>GSHMSAPLPLDELRTFAEVLDRVKAAYVEPVDDKTLLENAIKGMLSNLDPHSAYLGPEDFAELQESTSGEFGGLGIEVGSEDGFIKVVSPIDDTPAARAGIQPGDLIVQIDGKPTKGQSMTEAVDSMRGKAGSPITLTIVRDGGRPFDVELKRAIIKVKSVKSQVLEPGYAYLRITQFQVNTGEEVVKALNQLRKDNKGRLKGLVLDLRNNPGGVLQSAVEVADAFLTKGLIVYTKGRIANSELRFSADPADPSDKVPLVVLINGGSAAAAEIVAGALQDQKRAILMGTDSFGKGSVQTVLPLNNDRALKLTTALYYTPNGRSIQAQGIVPDIEVGRAKVTQERSSFEGFKEADLQGHLANGNGGADRPTGKRAAPSERPQDSDYQLSQALSLLKGLSVTRGN[6x];>MEDTAVETKAKPEKYGSFSEDSLYSLLVAELAGQRNRFDIALSNYVVQAQKTRDPGVSERAFRIAEYLGADQEALDTSLLWARSAPDNLDAQRAAAIQLARAGRYEESMVYMEKVLNGQGDTHFDFLALSAAETDPDTRAGLLQSFDHLLKKYPNNGQLLFGKALLLQQDGRPDEALTLLEDNSASRHEVAPLLLRSRLLQSMKRSDEALPLLKAGIKEHPDDKRVRLAYARLLVEQNRLDDAKAEFAGLVQQFPDDDDLRFSLALVCLEAQAWDEARIYLEELVERDSHVDAAHFNLGRLAEEQKDTARALDEYAQVGPGNDFLPAQLRQTDVLLKAGRVDEAAQRLDKARSEQPDYAIQLYLIEAEALSNNDQQEKAWQAIQEGLKQYPEDLNLLYTRSMLAEKRNDLAQMEKDLRFVIAREPDNAMALNALGYTLADRTTRYGEARELILKAHKLNPDDPAILDSMGWINYRQGKLADAERYLRQALQRYPDHEVAAHLGEVLWAQGRQGDARAIWREYLDKQPDSDVLRRTIKRLTGAETP[3x]

During bacterial cell growth, hydrolases cleave peptide cross-links between strands of the peptidoglycan sacculus to allow new strand insertion. The Pseudomonas aeruginosa carboxyl-terminal processing protease (CTP) CtpA regulates some of these hydrolases by degrading them. CtpA assembles as an inactive hexamer composed of a trimer-of-dimers, but its lipoprotein binding partner LbcA activates CtpA by an unknown mechanism. LbcA has an N-terminal adaptor domain that binds to CtpA, and a C-terminal superhelical tetratricopeptide repeat domain.

To address this question, we further refined the class IV EM map in which all three LbcA molecules are on the front side of the CtpA hexamer, which enabled the application of the C3 symmetry to improve the map quality and resolution. We improved the map to an overall resolution of 3.9 Å. We found that the movements of the PDZ domain, the core domain, and the NDR of the active CtpA in the LbcA-bound CtpA hexamer are comparable to those observed in the locally refined LbcA–CtpA dimer complex. However, the threefold symmetric complex structure reveals that the CDR helix H8 (aa 419–433) of the active CtpA shifts up by one helical turn, in response to the large changes in the upper region. These changes help maintain the trimer-of-dimers configuration of the CtpA complex bound to three LbcA. We found that the long loop (aa 376–411) that is disordered in the CtpA-alone hexamer structure becomes ordered in the LbcA–CtpA complex structure, and we now call it the trans-interacting loop (TIL). In the back view of the complex structure, the TIL loop from the inactive CtpA’ of the lower left CtpA dimer projects upward and inserts into a space in the top CtpA dimer between the PDZ of the inactive CtpA’ and the core domain of the active CtpA. Analysis of the structural features of TIL showed that the TIL Glu-385’ and Asn-394’ hydrogen bond with the active site His-84 and Gln-360, respectively. In addition to the polar interactions, the TIL residues Phe-383’ and Leu-388’ form a hydrophobic cluster with Phe-325 of the activated CtpA and Pro-147 of the inactive PDZ. As the TIL is specific for CtpA and is ordered only in the CtpA hexamer bound to three LbcA, it is likely that the loop’s function is primarily related to the active CtpA hexamer.Acetylxylan esterase from Caldanaerobacter subterraneus subsp. tengcongensis (TTE0866) has an N‐terminal region (NTR; residues 23–135) between the signal sequence (residues 1–22) and the catalytic domain (residues 136–324), which is of unknown function. Based on sequence and secondary structure analyses, NTR was confirmed to be an intrinsically disordered region. The crystal exhibited crystallographic properties comparable with those of the WT crystals suitable for structural determination. These results suggest that NTR plays a role in maintaining the solubility and inhibiting the crystallization of the catalytic domain.

Our previous study revealed the crystal structure of the wild‐type (WT) enzyme containing the NTR and the catalytic domain. Although the structure of the catalytic domain was successfully determined, that of the NTR was undetermined, as its electron density was unclear. In this study, we investigated the role of the NTR through functional and structural analyses of NTR truncation mutants. The truncation of NTR significantly decreased the solubility of the proteins at low salt concentrations compared with that of the WT. The NTR‐truncated mutant easily crystallized in a conventional buffer solution.

> GPAFSKKVLGSNPSSGKEVALTFDDGPFPIYTEKYVDILKSMDVKATFFVIGKHAEKHPELLKYIVENGNEIGLHSYSHFNMKKLKPEKMVEELYKTQQIIVEATGIKPTLFRPPFGAYNSTLIEISNALGLKVVLWNVDPDDWRNPSVESVVNRVLSHTRDGSIILMHEGKPSTLAALPQIIKKLKEEGYKFVTVSELLEKRD> MAAGVPCALVTSCSSVFSGDQLVQHILGTEDLIVEVTSNDAVRFYPWTIDNKYYSADINLCVVPNKFLVTAEIAESVQAFVVYFDSTQKSGLDSVSSWLPLAKAWLPEVMILVCDRVSEDGINRQKAQEWCIKHGFELVELSPEELPEEDDDFPESTGVKRIVQ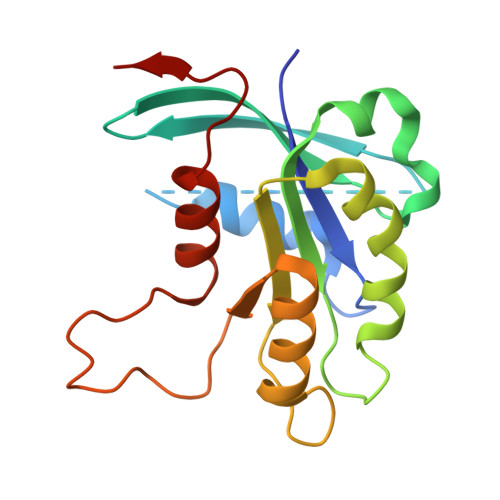ALNANVWSNVVMK>SGADTGAGAGMFRALFRQAVEDDRYGEFLDVLAEASAFRPQFASPEACSERLDPVLLAGGPTDRAEGRAVLVGCTGTAANGGPHEFLRLSTSFQEERDFLAVPL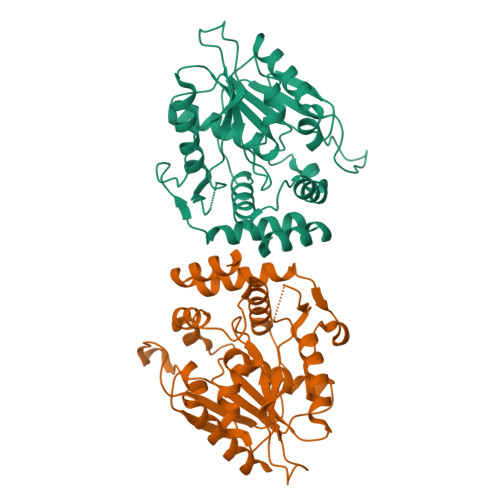PGYGTGTGTGTALLPADLDTALDAQARAILRAAGDAPVVLLGHSGGALLAHELAFRLERAHGAPPAGIVLVDPYPPGHQEPIEVWSRQLGEGLFAGELEPMSDARLLAMGRYARFLAGPRPGRSSAPVLLVRASEPLGDWQEERGDWRAHWDLPHTVADVPGDHFTMMRDHAPAVAEAVLSWLDAIEGIEGAGK[2x]>MNHKVHHHHHHLQENLYFQGMGAEPQQLHVVFFPIMAHGHMIPTLDIARLFAARNVRATIITTPLNAHTFTKAIEMGKKNGSPTIHLELFKFPAQDVGLPEGCENLEQALGSSLIEKFFKGVGLLREQLEAYLEKTRPNCLVADMFFPWATDSAAKFNIPRLVFHGTSFFSLCALEVVRLYEPHKNVSSDEELFSLPLFPHDIKMMRLQLPEDVWKHEKAEGKTRLKLIKESELKSYGVIVNSFYELEPNYAEFFRKELGRRAWNIGPVSLCNRSTEDKAQRGKQTSIDEHECLKWLNSKKKNSVIYICFGSTAHQIAPQLYEIAMALEASGQEFIWVVRNNNNNDDDDDDSWLPRGFEQRVEGKGLIIRGWAPQVLILEHEAIGAFVTHCGWNSTLEGITAGVPMVTWPIFAEQFYNEKLVNQILKIGVPVGANKWSRETSIEDVIKKDAIEKALREIMVGDEAEERRSRAKKLKEMAWKAVEEGGSSYSDLSALIEELRGYHA[2x]

PaGT3, a uridine diphosphate glycosyltransferase (UGT) from Phytolacca americana, is known for its ability to glycosylate capsaicinoids and other phenolic compounds. PaGT3 adopts a GT-B-fold structure that is highly conserved among UGTs. However, the acceptor-binding pocket in PaGT3 is hydrophobic and large, and is surrounded by longer loops. The larger acceptor-binding pocket in PaGT3 allows the enzyme to bind a range of compounds, while the flexibility of the longer loops possibly plays a role in accommodating the acceptors in the binding pocket according to their shape and size.

The crystal structure of PaGT3 with the sugar-donor analogue UDP-2FGlc was determined at 2.20 Å resolution. UDP-2FGlc occupies the sugar-donor binding cavities in all three PaGT3 crystal structures. Compared with the apo PaGT3 structure the same loop is seen to shift outwards in the UDP-2FGlc-bound structure, and it shifts further outwards in the capsaicin-bound structure due to the binding of the larger capsaicin molecule. The loops Cys289–Ile297 and Val412–Lys429 shift towards the pocket in the substrate-bound structures compared with the apo PaGT3 structure. In the substrate-bound PaGT3 structures, the indole moiety of Trp352 flips ∼180° to form a π-stacking interaction with the uracil ring of the sugar-donor analogue. Similarly, the side chain of His370 rotates ∼120° to form a hydrogen bond to the O3A atom on the α-phosphate moiety of UDP-2FGlc. The side chain of His18 is likely to contribute to stabilizing the sugar moiety by forming a hydrogen bond to the 6-OH of 2-fluoroglucose. His18, Gly19 and Glu87 stabilize the sugar-donor analogue through water-mediated hydrogen bonds.>CGCGUG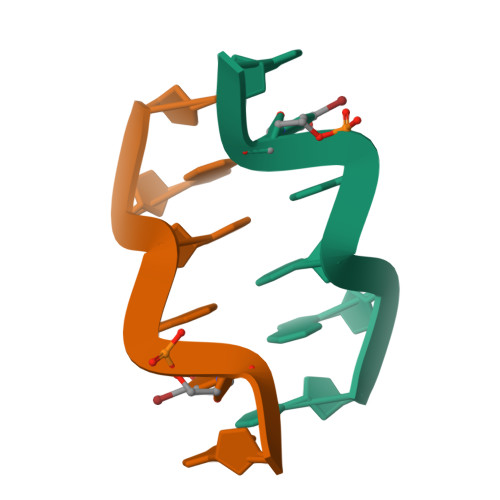[2x]>[2x]MGGEIITLQAGQCGNHVGKFLWSQLAKEHAIGTDGLSQLPDSSTERDDDTKPFFRENSRNKFTPRAIMMDSEPSVIADVENTFRGFFDPRNTWVASDGASAGNSWANGYDIGTRNQDDILNKIDKEIDSTDNFEGFQLLHSVAGGTGSGLGSNLLEALCDRYPKKILTTYSVFPARSSEVVVQSYNTILALRRLIEDSDATVVFDNASLLNISGKVFRNPNIDLQHTNQLISTIISSVTNSIRFPSYMYSSMSSIYSTLIPSPELHFLSPSFTPFTSDYIHDDIAHKGHSSYDVMLDLLDPSNSLVSTAMNNPTYFNVYNTIIGNVEPRQISRAMTKLQQRIKFPSWSSSAMHVNIGRRSPYLPLQPNENEVSGMMLSNMSTVVNVFENACNTFDKVFAKGAFLNNYNVGDLFQSMQNVQDEFAESREVVQSLMEDYVAAEQDSYLDDVLVDDENMVGELEEDLDADGDHKLV;> MELEPTLFGIIEALAPQLLSQSHLQTFVSDVVNLLRSSTKSATQLGPLIDFYKLQSLDSPETTIMWHKIEKFLDALFGIQNTDDMVKYLSVFQSLLPSNYRAKIVQKSSGLNMENLANHEHLLSPVRAPSIYTEASFENMDRFSERRSMVSSPNRYVPSSTYS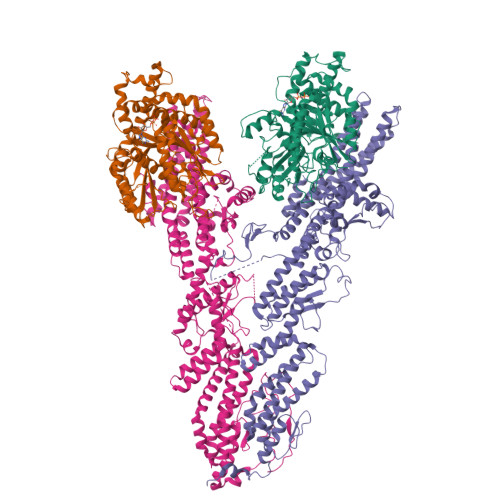SVTLRQLSNPYYVNTIPEEDILKYVSYTLLATTSALFPFDHEQIQIPSKIPNFESGLLHLIFEAGLLYQSLGYKVEKFRMLNISPMKKALIIEISEELQNYTAFVNNLVSSGTVVSLKSLYREIYENIIRLRIYCRFTEHLEELSGDTFLIELNIFKSHGDLTIRKIATNLFNSMISLYYEYLMNWLTKGLLRATYGEFFIAENTDTNGTDDDFIYHIPIEFNQERVPAFIPKELAYKIFMIGKSYIFLEKYCKEVQWTNEFSKKYHVLYQSNSYRGISTNFFEIINDQYSEIVNHTNQILNQKFHYRDVVFALKNILLMGKSDFMDALIEKANDILATPSDSLPNYKLTRVLQEAVQLSSLRHLMNSPRNSSVINGLDARVLDLGHGSVGWDVFTLDYILYPPLSLVLNVNRPFGRKEYLRIFNFLWRFKKNNYFYQKEMLKSNDIIRSFKKIRGYNPLIRDIINKLSRISILRTQFQQFNSKMESYYLNCIIEENFKEMTRKLQRTENKSQNQFDLIRLNNGTIELNGILTPKAEVLTKSSSSKPQKHAIEKTLNIDELESVHNTFLTNILSHKLFATNTSEISVGDYSGQPYPTSLVLLLNSVYEFVKVYCNLNDIGYEIFIKMNLNDHEASNGLLGKFNTNLKEIVSQYKNFKDRLYIFRADLKNDGDEELFLLSKSLR;> MEIKEVDDRAELLRYTNNIPLLGKLVNHQPLWSTNPKLKSFSLEKISAPDQRRVQEALVVKDLLNVLIGLEGTYIRYFNDYEPSDPETPIEFKIAKKMDPSFKTFSRRIVRYGKQYMILTRAYEKWSDTSFGMVLQRFAYEIRRFLEDVYLKTLVERLERDFNKVPNFSIRELEQIINETEVNKQMELLYNIYEEIFREIEERRTNQSSQEDFNNFMDSMKNESSLHLRLMVAFDTTVYPVPKGGAILKIFQQKILENLGDRSSVMFLKKLLNNISQDYCTMLYEWLTQGILNDPYQEFMTYDDLEGKTDNIFDTRDRAWDTQYFIRKDVLLRDCDSEEDKNLLFKMLRTGILLKVVRASLQIPTIPSNSSDITIQEINDFADLMEGSNLELYVDKCYSRANEIFLKLFFQGYDLINVLKHLQQIFLGYQSGHNVLKFLTKNMGELTKHYRNDNNANYDKLLQNFELERQSENPNNLMRQLLMIQFDTETLPQVLSHYLQIYPEVPENNSANDDSDPLMHANNFKNMNAILFDELSKERTGAYHGSNLELYTPKSAIYHLKFDINIPYPLNIIISRTCMIKYQIILRYQLVLQYHSRLLDETWMDLNKTPSWKYRGYSHTVKRRIVRATRVLHAKMNHFIKTIMEYFNQNVIDKEVYSLEKCYRNPTLAVAIQNELEGGLTNIMTNRCLSDLIPLQLQIFDIVYKFCKFIKSMRAKLCQLDPVLYEKHKSGMMKTLNEGYRTNNGGQEDVGYQEDAALELIQKLIEYISNASSIFRKCLINFTQELSTEKFDFYDSSSVDAAGIERVLYSIVPPRSASASSQR N-[(cyclopropylamino)(oxo)acetyl]-beta-D-glucopyranosylamine 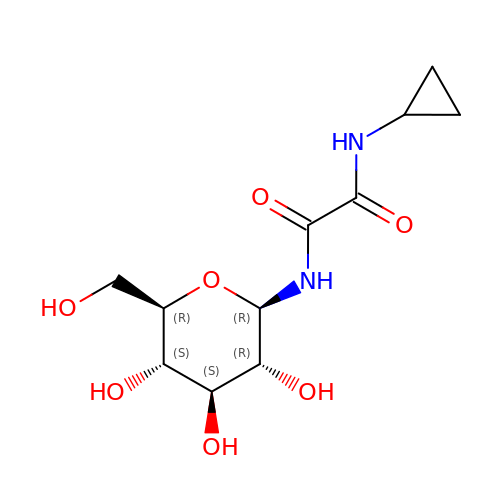| C11 H18 N2 O7 | ZDEMZENRHYGLSV-NEBGFLKFSA-N> MEQKLISEEDLGGGEQKLISEEDLGGGEQKLISEEDLGGGMDKDCEMKRTTLDSPLGKLELSGCEQGLHRIIFLGKGTSAADAVEVPAPAAVLGGPEPLIQATAWLNAYFHQPEAIEEFPVPALHHPVFQQESFTRQVLWKLLKVVKFGEVISESHLAALVGNPAATAAVNTALDGNPVPILIPCHRVVQGDSDVGPYLGGLAVKEWLLAHEGHRLGKPGLGGGSGMATRGANVIWFRHGLRLHDNPALLAALADKDQGIALIPVFIFDGESAGTKNVGYNRMRFLLDSLQDIDDQLQAATDGRGRLLVFEGEPAYIFRRLHEQVRLHRICIEQDCEPIWNERDESIRSLCRELNIDFVEKVSHTLWDPQLVIETNGGIPPLTYQMFLHTVQIIGLPPRPTADARLEDATFVELDPEFCRSLKLFEQLPTPEHFNVYGDNMGFLAKINWRGGETQALLLLDERLKVEQHAFERGFYLPNQALPNIHDSPKSMSAHLRFGCLSVRRFYWSVHDLFKNVQLRACVRGVQMTGGAHITGQLIWREYFYTMSVNNPNY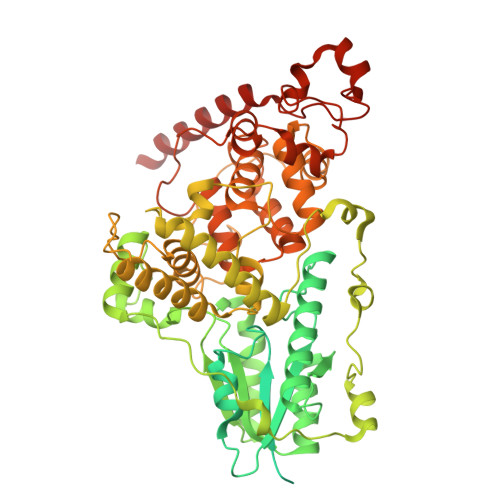DRMEGNDICLSIPWAKPNENLLQSWRLGQTGFPLIDGAMRQLLAEGWLHHTLRNTVATFLTRGGLWQSWEHGLQHFLKYLLDADWSVCAGNWMWVSSSAFERLLDSSLVTCPVALAKRLDPDGTYIKQYVPELMNVPKEFVHEPWRMSAEQQEQYECLIGVHYPERIIDLSMAVKRNMLAMKSLRNSLITPP propan-2-yl 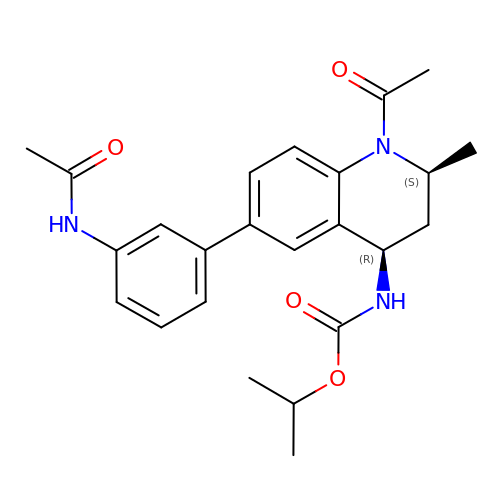~{N}-[(2~{S},4~{R})-6-(3-acetamidophenyl)-1-ethanoyl-2-methyl-3,4-dihydro-2~{H}-quinolin-4-yl]carbamate | C24 H29 N3 O4 | UIHJJMSWZNYBQU-OYHNWAKOSA-N> EAIPRSIPPEVKFNKPFVFLMIEQNTKSPLFMGKVV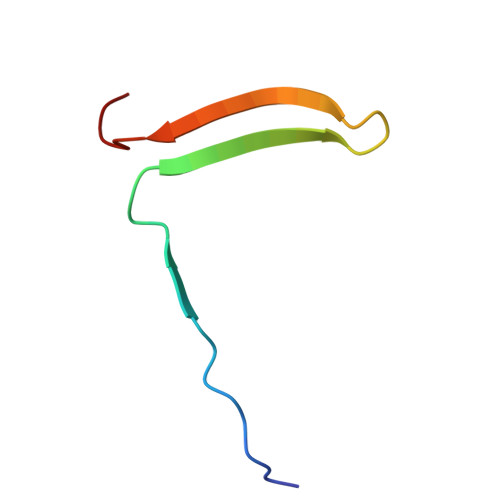NPTQK> GAMSTLGDLLAEHTVLPGSAVDHLHAVVGEWQLLADLSFADYLMWVRRDDGVLVCVAQCRPNTGPTVVHTDAVGTVVAANSMPLVAATFSGGVPGREGAVGQQNSCQHDGHSVEVSPVRFGDQVVAVLTRHQPELAARRRSGHLETAYRLCATDLLRMLAEGTFPDAGDVAMSRSSPRAGDGFIRLDVDGVVSYASPNALSAYHRMGLTTELEGVNLIDATRPLISDPFEAHEVDEHVQDLLAGDGKGMRMEV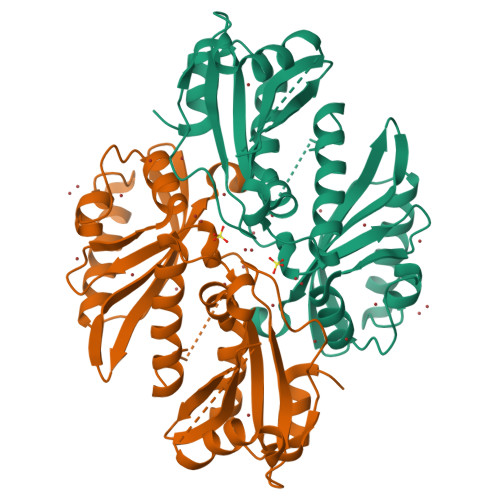DAGGATVLLRTLPLVVAGRNVGAAILIRDVTEVKRRDRALISKDATIREIHH>[2x]MATVEPETTPTPNPPTTEEEKTESNQEVANPEHYIKHPLQNRWALWFFKNDKSKTWQANLRLISKFDTVEDFWALYNHIQLSSNLMPGCDYSLFKDGIEPMWEDEKNKRGGRWLITLNKQQRRSDLDRFWLETLLCLIGESFDDYSDDVCGAVVNVRAKGDKIAIWTTECENREAVTHIGRVYKERLGLPPKIVIGYQSHADTATKSGSTTKNRFVV;>XKKRYSREFLLGFX[2x]

eIF4E initiates cap-dependent translation by binding to the cap structure (m7GTP) found at the 5′ end of mRNA. eIF4E is part of the large eIF4F complex which includes other proteins such as eIF4G and eIF4A. eIF4F forms a complex with the 40S ribosomal subunit and eIF3, which then shuttles along the 5′-untranslated region (5′-UTR) of the mRNA until it arrives at the AUG initiation codon. The interaction of eIF4E with eIF4G, as part of the eIF4F complex, is competitively blocked by the binding of the 4E-binding proteins (4E-BPs) to eIF4E. The 4E-BP1 and eIF4GI peptides both posses a YXXXXLΦ motif (Φ signifies any hydrophobic residue). In this study we isolated a novel phage derived peptide against eIF4E and identified two amino acid positions outside the conserved interaction motif that improved binding of the eIF4G1 sequence.

Interestingly there were two key substitutions that improved the affinity of the eIF4G1 sequence, a D to S substitution at position 5 and a G to A substitution at position 11. The D5S substitution caused an apparent 4.6-fold improvement in binding to eIF4E whilst the G11A mutation caused an ∼ 2.3-fold improvement. eIF4E was successfully crystallized with the eIF4G1_D5S peptide which revealed the mechanism for the improvement in its affinity over the wild type peptide for this mutation. The hydroxyl group of the serine forms two optimal hydrogen bonds with the amide backbone groups of E7 and F8, which form the initial turn of the peptide α-helix seen in the crystal structure. The amide backbone groups in the first turn of the α-helix are not involved in hydrogen bonds with other residues in the helix and as a result are responsible for the positive dipole found at the N-terminal of helices. The two hydrogen bonds formed by the hydroxyl group of the serine with the first turn of the helix are slightly shorter and hence energetically more favorable (3.2 and 3.4 Å respectively) when compared to the eIF4G1 peptide (3.3 and 3.5 Å respectively) in the crystal structures. In the alternative complexes in the asymmetric unit of both structures the bonds distances are 3.0 Å and 3.5 Å for the S5 modification compared to 3.5 Å and 4.4 Å for the D5 residue, respectively. In the simulation of the eIF4G1 wild-type peptide, the D5 side chain occasionally forms hydrogen bonds with the R186 side chain of eIF4E, causing a slight deformation at the N-terminal end of the α-helix in the bound peptide. When the capping residue D5 is changed to S5 in the eIF4G1_D5S peptide, the deformation appears to be attenuated. This results in greater stabilization of E132 of eIF4E with R6 of the peptide, leading to improved interactions of the peptide with eIF4E.To understand the structure and function of the C. difficile eut bacterial microcompartment we have determined the crystal structures of two proteins with homology to BMC shell proteins, CD1908 and CD1918, and show that they are well conserved between species. We have also determined the atomic structure of CD1925, a member of the EutQ family of cupin barrels. The sequestration of ethanolamine metabolism within a BMC is thought to protect the cell from the acetaldehyde produced as an intermediate in its breakdown and to prevent the loss of this volatile compound and its carbon from the cell.

The crystal structure of a CD1925 variant, truncated at the N-terminus by 16 amino acids (CD1925(17–157)), was solved by molecular replacement and determined to 1 Å resolution. Two chains were present in the asymmetric unit, with residues 28–153 visible in chain A and 29–157 visible in chain B, with the majority of the C-terminal His6 tag also visible in the latter chain. The protein belongs to the EutQ family of cupins and has the distinct β-barrel fold associated with these proteins. The two chains in the asymmetric unit form a dimer, with a total interface area of 1740 Å2 out of 9285 Å2 total surface area for each monomer. This dimer interface is formed between one face of the β-barrel of each monomer, with an interaction between β9 of one monomer and β2 of the partner chain, thus extending the β-sheet across the two molecules. The surface of CD1925 does not display the distinctive charge distribution patterns seen for the oligomeric BMC proteins CD1908 and CD1918; instead its surface has irregular patches of positive and negative electrostatic potential. A shallow, negatively charged cleft is visible on the surface of each protein chain within the cupin β-barrel (Fig. 6B white oval), this cleft corresponds to the region that coordinates divalent cations and acts as the active site in the metal binding cupins, such as those with sugar isomerase activity (Fig 7A/B). In contrast to the metal-binding catalytic cupins, CD1925 and the EutQ family, do not possess the histidine residues that are responsible for metal coordination in the oxidoreductase and epimerase classes of cupins. In the place of the histidine residues are aromatic (Trp94) and hydrophobic residues (Leu 96, Ile134) and in the fourth position a glutamic acid residue (Glu100) (Fig. 7B/C), which is also present in the cupins with epimerase activity. The glutamic acid (Glu100) is within hydrogen bonding distance of an aspartic acid residue (Asp102), which may act to alter its pKa. Because of strong sequence conservation seen in this area for the EutQ family and the fact that this region is solvent accessible and it corresponds with the position of the catalytic site of other cupins, this region may act to bind ligands, or act as a catalytic centre (starred residues).

>MGQIIEEKISGTKDTVDFVRNKDISGITSIKLPTVKVSESDRLDTGNPSDVVYTKDLFTLEESPRLGCGMMEMKETTFDWTLNYDEIDYVIDGTLDIIIDGRKVSASSGELIFIPKGSKIQFSVPDYARFIYVTYPADWASQNLEHHHHHH[2x]> MEHVAFGSEDIENTLAKMDDGQLDGLAFGAIQLDGDGNILQYNAAEGDITGRDPKQVIGKNFFKDVAPCTDSPEFYGK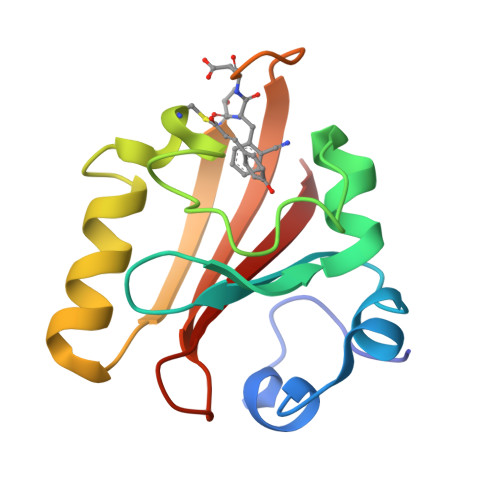FKEGVASGNLNTMFEYTXDYQQTPTKVKVHMKKALSGDSYWVFVKRV> GHMSLSVAEKSYLYDSLASTPSIRPDGRLPHQFRPIEIFTDFLPSSNGSSRIIASDGSECIVSIKSKVVDHHVENELLQVDVDIAGQRDDALVVETITSLLNKVLKS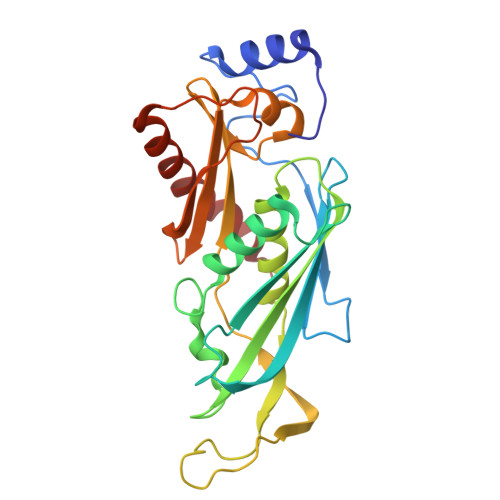GSGVDSSKLQLTKKYSFKIFVDVLVISSHSHPISLISFAIYSALNSTYLPKLISAFDDLEVEELPTFHDYDMVKLDINPPLVFILAVVGNNMLLDPAANESEVANNGLIISWSNGKITSPIRSVALNDSNVKSFKPHLLKQGLAMVEKYAPDVVRSLENL(2M)-4'-methyl-2-(2H-tetrazol-5-yl)[1,1'-biphenyl]-3-sulfonamide | C14 H13 N5 O2 S | 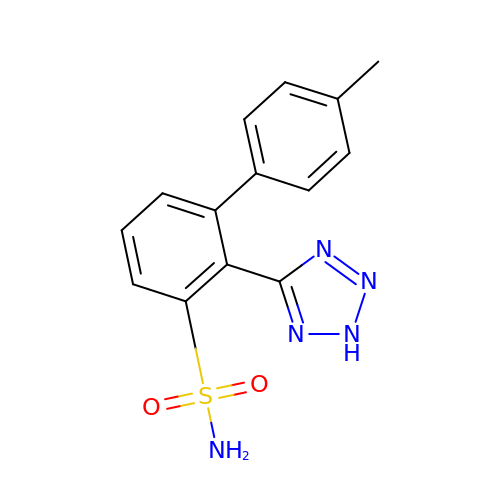JNVRWMYBFOXGPS-UHFFFAOYSA-N> GSQLRGEPWFHGKLSRREAEALLQLNGDFLVRESTTTPGQYVLTGLQSGQPKHLLLVDPEGVVRTKDHRFESVSHLISYHMDNHLPII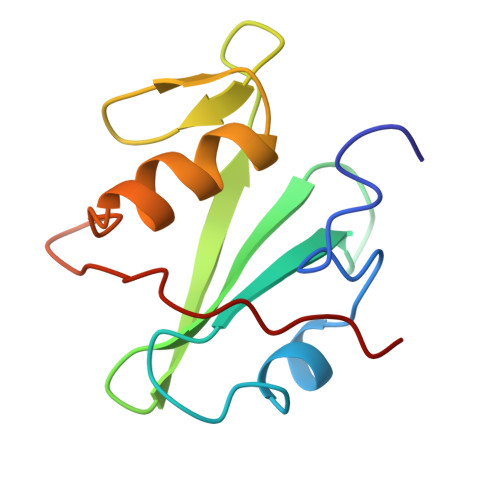SAGSELCLQQPVERKL(2R)-2-(4-cyclohexylnaphthalen-1-yl)propanoic acid | 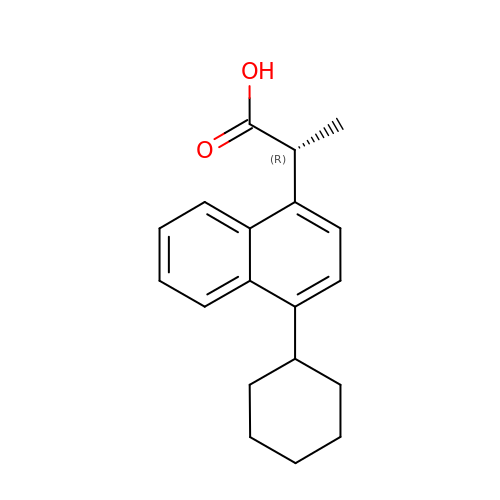C19 H22 O2 | VZUGVMQFWFVFBX-CYBMUJFWSA-N Here, we report the structure and kinetic rate parameters for a glycoside hydrolase (GH) family 5 subfamily 4 enzyme (CelD) from Piromyces finnis, a modular, cellulosome-incorporated endoglucanase that possesses three GH5 domains followed by two C-terminal fungal dockerin domains (double dockerin). In this study, we characterized, at the structural and functional levels, the CelD enzyme from the anaerobic fungus Piromyces finnis. This fungal enzyme belongs to the glycoside hydrolase (GH) family 5 subfamily 4 of cellulases and acts strictly as an endo-β-1,4-glucanase (EC 3.2.1.4) with confirmed activity against carboxymethylcellulose (CMC), mixed linkage glucan (MLG), and xyloglucan. The CelD catalytic domain displays strong structural similarity to GH clan A, a group of 28 unique GH families exhibiting a (β/α)8–barrel fold in structure, with the highest sequence similarity to proteins from GH5 subfamily 4 (GH5_4), a family of enzymes that predominantly display endoglucanase activity (EC 3.2.1.4). Like other GH5 enzymes, CelD contains two invariant catalytic glutamate residues, the acid/base Glu154 and the nucleophile Glu278.

Attempts to crystallize the CelD active catalytic domain with cellobiose or cellotriose substrates were unsuccessful using both soaking and co-crystallization approaches. After introducing the inactivating E154A mutation to the active site of a single CelD catalytic domain, we were able to obtain high-quality crystals of the E154A-cellotriose complex. The unliganded structures of the wild-type catalytic domain and its inactive E154A mutant in complex with cellotriose were determined by molecular replacement and refined to 2.5 Å and 1.8 Å resolution, respectively. Superposition of two structures solved in this work confirms that the carboxylate OE1 and OE2 oxygens of the catalytic acid/base glutamate point towards the O1 atom of the − 1 glucopyranose unit at 1.5 Å and 1.7 Å, respectively, and the carboxylate oxygen of the complementary nucleophile glutamate forms a hydrogen bond with the anomeric C1 carbon of the same saccharide unit at 3.1 Å. Meanwhile, the nucleophile Glu278 is sandwiched between two conserved Arg66 and Tyr231 residues which form hydrogen bonds to the carboxylate oxygens and appear to serve a supportive role to stabilize this Glu residue throughout catalysis as observed for other GH5 enzymes. We found 8 ordered water molecules making multiple hydrogen bonds with both the protein moiety and the cellotriose molecule in the ligand-bound structure; two of them are located near the anomeric carbon of the − 1 saccharide moiety. One of these water molecules may participate in the catalytic mechanism of the CelD as a nucleophilic attack on the glycosyl-enzyme intermediate.

>[2x]SNAIRDISSIELIKEMRFGWNLGNTLDAECTSWMDYEKNPIGSETCWGNVKTNEDIFKTLMDNQFNVFRIPTTWTGHIGEAPEYKINEQWMKRVHEIVDYPYKNGAFVILNIHHETWNHAFAETVDEAKVELAQVWKQIAEEFKGYGERLIFEGQNAPRKNGTPVEWNGGDKEGWDVVNAMNAVFLETVRSSGGNNAKRHLMIPPYAAACNENSFKNFDFPEDDDKVIASVHAYSPYNFALNNGEGAVDKFDASGKNELDWNINLMKKRFVDQGIPMILGEYGAMNRDNEEERAAWAEYYMEKITALGVPQVWWDNGVFEGEGERFGLIDRKNLKIVYPSIVAALQKGRGLEVNVLHAIETEPEE>HDDRRTLWTTPDPSPNCTIDEERDSKLTLVLTKCGSQILANVSLLVVKGKFSNINNNTNPTDKKITVKLLFNEKGVLMDSSSLKKEYW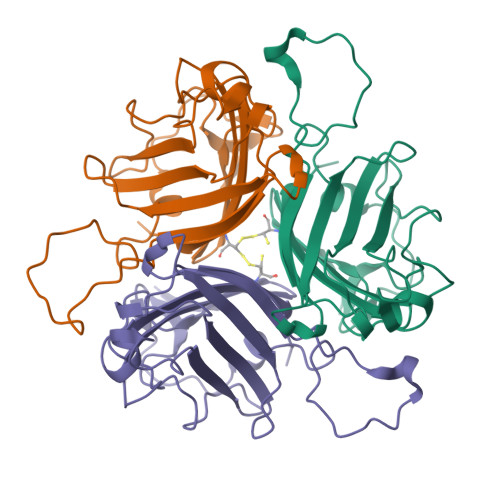NYRNDNSTVSQAYDNAVPFMPNIKAYPKPTTDTSAKPEDKKSAAKRYIVSNVYIGGLPDKTVVITIKLNAETESAYSMTFEFTWAKTFENLQFDSSSFTFSYIAQEN[3x]> MGSSHHHHHHSSGENLYFQGMPEESSPR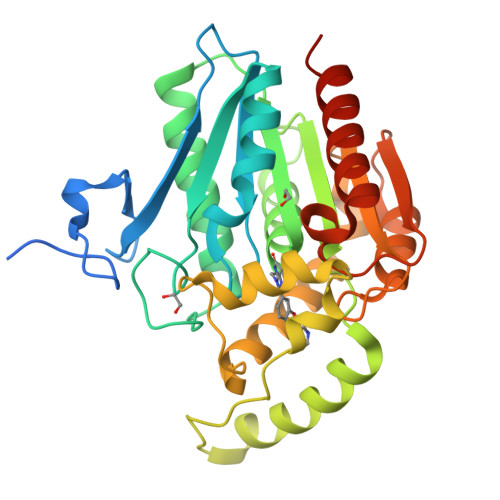RTPQSIPYQDLPHLVNADGQYLFCRYWAPTGTPKALIFVSHGAGEHSGRYEELARMLMGLDLLVFAHDHVGHGQSEGERMVVSDFHVFVRDVLQHVDSMQKDYPGLPVFLLGHSMGGAIAILTAAERPGHFAGMVLISPLVLANPESATTFKVLAAKVLNSVLPNLSSGPIDSSVLSRNKTEVDIYNSDPLICRAGLKVCFGIQLLNAVSRVERALPKLTVPFLLLQGSADRLCDSKGAYLLMELAKSQDKTLKIYEGAYHVLHKELPEVTNSVFHEINMWVSQRTATAGTASPP> VAFGADAAKTTQEKFDALKEAGVFSGYPGTTDAKLGQDMTRAEFAKVLVKLFGLKEIHGQYSYKDKNYDAKNWAAPFIEAVTA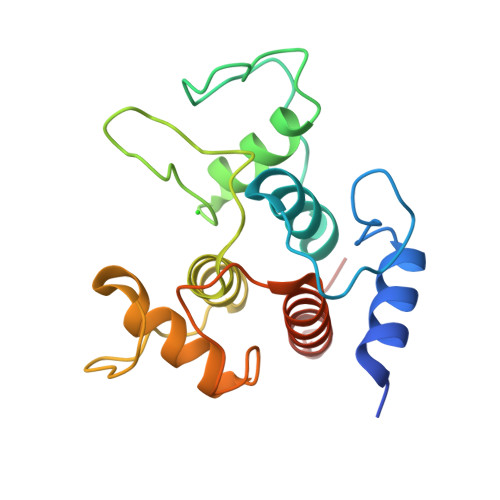EGLMQAKDLTKKIFDFNGKITVEEASKTLVTALKLEPVKDAQNKATDWAKGYFEAAVNAGLFSKDANPKANATRAQLVEAAFAADEMSKGSGSHHHHHH> MLLKNAVQLICYPDRIGNNLKDLYTVVDTHLSEAIGGLHILPFFPSNADGGFSPLTHKEVDPKFGTWDDIEAFTAKYDLCVDLTVNHISDESPEFKDFIANGFDSEYADLFVHVDKFGEISPDDLALIHIRKEKEPFREVTLADGTKTRVWCTFTEQQIDLNYESPLAYQLMESYIGFLTSKGVNLLRLDAFGYTTKRIGTSCFLVEPEVYQILDWINQVALKHGAECLPEVHDHISYQYAISRRNMHPYGFALPPLLLYSLLDANSTYLKNWLRMCPRNMVTVLDTHDGICIPDVEGVLPDEKIKVLIDNIDARSADPIMRRSAANIHSVGAI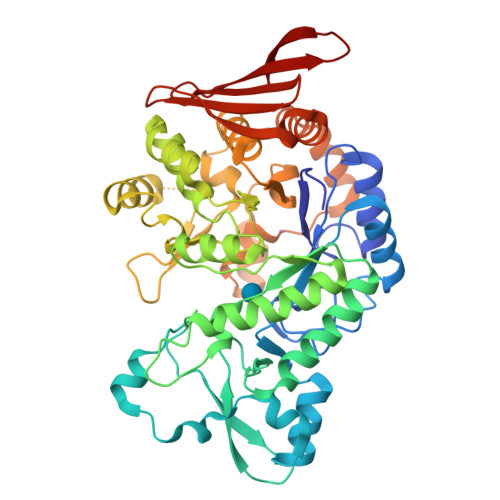YQLTCTFYDALMQNDDAYIAARAIQFFTPGIPQVYYVGLLAGCNDHELMEQTGELRDINRHYYTLEEVEQDIQKPVVQRLLSLMKFRSNYPAFDGHFELNYSNNSSVAMAWRHGDYYCHLFVDLNFKTVKVTYTDVETGETRHLEC>[3x]MHHHHHHHHENLYFQGSETPAEPKLPVVVEAHQVDTFDVPGVFYENHPHEPHLSGMNEYNQLYQQSINDPDTFWARMARDLITFEKDFDKTHIGTLEGGDNAWFVGGRLNASFNCVDRHAMRDPNKVAIIYEAD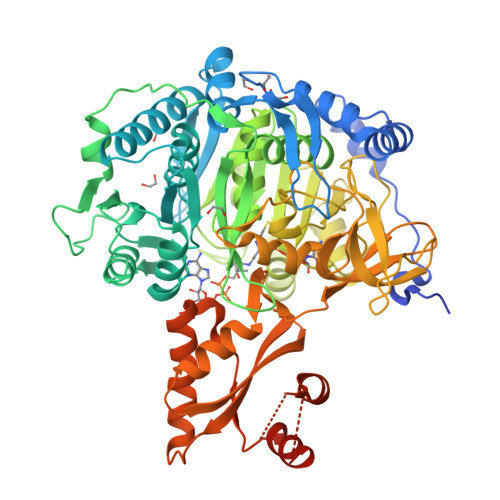EPGHGRSITYAELLKEVSRLAWVMKSQGVRKGDTVAIYLPMIPEAIFALLACARIGAIHSVVFAGFSSDSLRDRTLDARSKFIITTDEGKRGGKVIGTKKIVDEALKQCPDVTNCLVFKRTGADVPWTKGRDLWWHEEVDKYPNYLPAESMDSEDPLFLLYTSGSTGKPKGVMHTTAGYLVGAAATGKYVFDIHPADRFFCGGDVGWITGHTYVVYAPLLLGCTTVVFESTPAYPNFSRYWDVIEKHKVTQFYVAPTALRLLKRAGDHHINHEMKDLRILGSVGEPIAAEVWKWYHEVVGKRQAHIVDTYWQTETGSHVITPLGGITPTKPGSASLPFFGIDPVILDPVTGAEIPGNDVEGILAFRKPWPSMARTVWGDHKRYMDTYLNVYKGFYFTGDGAGRDHEGYYWIRGRVDDVVNVSGHRLSTAEIEAALIEHHCVAEAAVVGVPDPLTGQAVHAFVALKSGNDNREQLQKELIMQVRKSIGPFAAPKVVFVIDDLPKTRSGKIMRRILRKILSGEEDSLGDISTLSDPSVVNKIIDTFHEWKKAMAAAAAAAAAVSATAPPNSTTG(1R)-4-(3-phenoxyphenyl)-1-phosphonobutane-1-sulfonic acid | C16 H19 O7 P S | 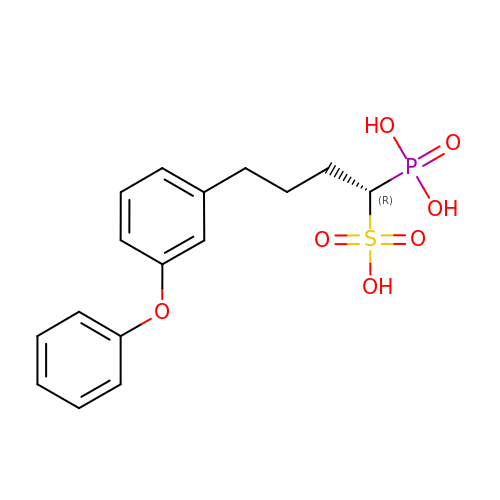RCGCZPXSRLLKCK-MRXNPFEDSA-N> MEHHHHHHTMLVYTEEDNISQLWGLYEMSREKLENDDIDASVSLVFGTIHEADRILRNTEDISTLPKDFHAAYSSALLAVSELFEIAQKRLKETNTEESYIDAAIERAQLGLDAPGNESRLFLALARAYLEKVRVLVWRHDNEESLANIPVTQLVNPY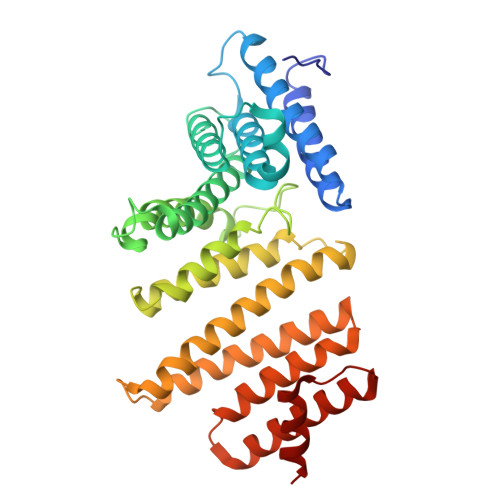IEKAIQYLRPLAQDSTEYFDALTPDSLRPLYILSSYLFQFGDQFSEAFLLDVCSIITALWLKSVVDPNTPAYYKLIAQEAVLNNYTTFAEYYMDLLDNSESNVDDLINKASSWLNNSVDTWNVIYTLDKSPERLLKLADIKMDLAQIVQDEASQDNYLKEACNAIKEAQGSGVELSPDYVEFVEAYSA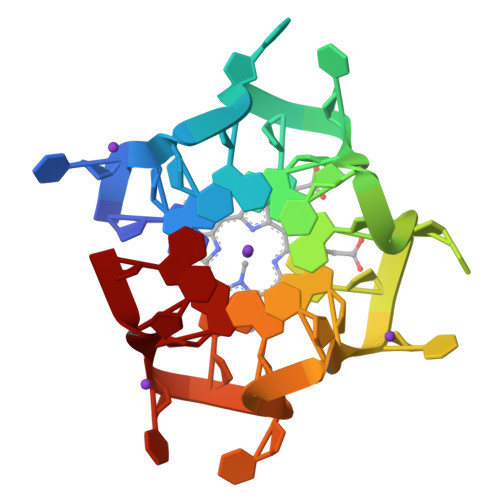> GUGUGUGUGUGUGUGUGUGUGUG> APDTSVSNKQNFSTDVIYQIFTDRFSDGNPANNPTGAAFDGTCTNLRLYCGGDWQGIINKINDGYLTGMGVTAIWISQPVENIYSIINYSGVNNTAYHGYWARDFKKTNPAYGTIADFQNLIAAAHAKNIKVIIAFAPNHTSPASSDQPSFAENGRLYDNGTLLGGYTNDTQNLFHHNGGTDFSTTENGIYKNLYDLADLNHNNSTVDVYLKDAIKMWLDLGIDGIRMDAVKHMPFGWQKSFMAAVNNYKPVFTFGEWFLGVNEVSPENHKFANESGMSLLDFRFAQKVRQVFRDNTDNMYGL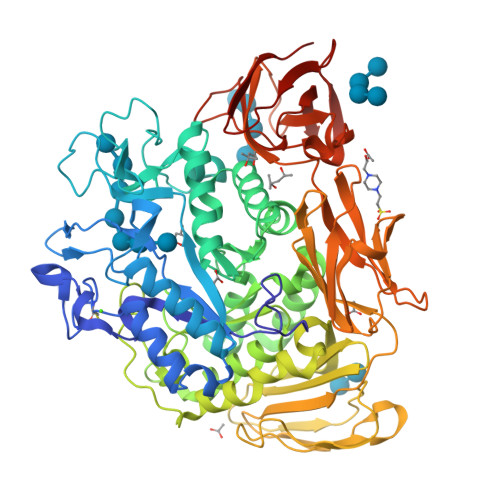KAMLEGSAADYAQVDDQVTFIDNHDMERFHASNANRRKLEQALAFTLTSRGVPAIYYGTEQYMSGGTDPDNRARIPSFSTSTTAYQVIQKLAPLRKSNPAIAYGSTQERWINNDVLIYERKFGSNVAVVAVNRNLNAPASISGLVTSLPQGSYNDVLGGLLNGNTLSVGSGGAASNFTLAAGGTAVWQYTAATATPTIGHVGPMMAKPGVTITIDGRGFGSSKGTVYFGTTAVSGADITSWEDTQIKVKIPAVAGGNYNIKVANAAGTASNVYDNFEVLSGDQVSVRFVVNNATTALGQNVYLTGSVSELGNWDPAKAIGPMYNQVVYQYPNWYYDVSVPAGKTIEFKFLKKQGSTVTWEGGSNHTFTAPSSGTATINVNWQP Pinoresinol/lariciresinol reductase (PLR), an NADPH-dependent reductase, converts pinoresinol to lariciresinol and subsequently to secoisolariciresinol. Here, we present crystal structures of IiPLR1 from Isatis indigotica and pinoresinol reductases (PrRs) AtPrR1 and AtPrR2 from Arabidopsis thaliana, in the apo, substrate-bound and product-bound states. The crystal structures were captured in the apo, substrate-bound and/or product-bound forms. We found that, for all 16 structures we solved, each enzyme adopts a similar head-to-tail dimer conformation, strongly suggesting that each PLR/PrR functions as a homodimer, consistent with the literature that TpPLR1 exists as a dimeric entity in solution. Each structure contains a head-to-tail homodimer, and the catalytic pocket comprises structural elements from both monomers. β4 loop covers the top of the pocket, and residue 98 from the loop governs catalytic specificity.

Each of IiPLR1_NAP_ + PIN/AtPrR1_NAP_ + PIN/AtPrR2_NAP_ + PIN forms a homodimer, and superimposition of the protomers among the three complexes revealed RMSDs of 0.374, 0.365, and 0.308 Å, respectively. In contrast to IiPLR1_NAP_ + PIN, the β4 loops of AtPrR1_NAP_ + PIN and AtPrR2_NAP_ + PIN can be clearly identified. These well-defined loops twist as an “8” shape and cover both the NADP+-binding and substrate-binding grooves. Within the twisted loop, His93 and His97 “grasp” helices α5 and α10, while Val92 and Phe94 interact directly with (+)-pinoresinol; Arg95 strongly interacts with NADP+ as well as each of the GXXGXXG motif and α2-helix from neighboring protomer of the dimer. Similar conformational changes of β2 loop and α10-helix can be seen by comparing the structure of AtPrR1_NAP_ + PIN with that of AtPrR1_NAP and the structure of AtPrR2_NAP_ + PIN with that of AtPrR2_apo. Furthermore, Leu46 (corresponding to Val46 in IiPLR1), His276 and Phe277 of AtPrR1 are positioned similar to the corresponding residues of IiPLR1 to effect substrate binding or product release, except that the β4 loops cover the substrate/product, which are disordered in the IiPLR1 structures. Besides the β4 loop, Val46 in IiPLR1 is replaced with Leu46 in AtPrR1, which has the effect of compressing the substrate-binding pocket. Therefore, the entrance and orientation of the substrate in AtPrR1/2 is more tightly controlled than in IiPLR1.

>MGESKRTEKTRVLVVGATGYIGKRIVRACLAEGHETYVLQRPEIGLEIEKVQLFLSFKKLGARIVEGSFSDHQSLVSAVKLVDVVVSAMSGVHFRSHNILVQLKLVEAIKEAGNVKRFLPSEFGMDPPRMGHALPPGRETFDQKMEVRQAIEAAGIPYTYVVGACFAAYFAGNLSQMVTLLPPKEKVNIYGDGNVKVVFADEDDIAKYTAKTLNDPRTLNKTVNIRPPDNVLTQLELVQIWEKLTGKELEKTNIAAQDFLANIEQMEIPHQAGIGHFYHIFYEGCLTDHEVGEDEEASSLYPDVKYKRMDDYLRMFL[4x]>[2x]MAAAAAEEGMEPRALQYEQTLMYGRYTQDLGAFAKEEAARIRLGGPEPWKGPPSSRAAPELLEYGRSRCARCRVCSVRCHKFLVSRVGEDWIFLVLLGLLMALVSWVMDYAIAACLQAQQWMSRGLNTSILLQ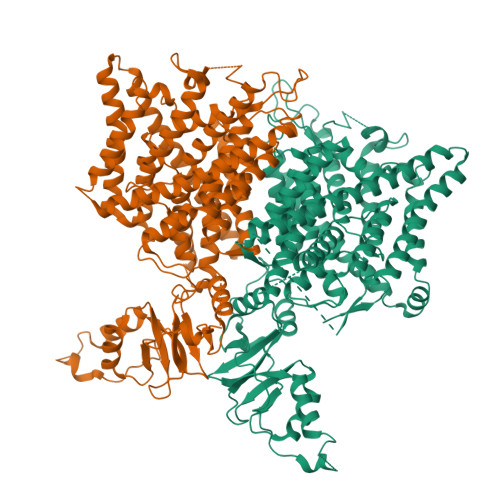YLAWVTYPVVLITFSAGFTQILAPQAVGSGIPEMKTILRGVVLKEYLTLKTFIAKVIGLTCALGSGMPLGKEGPFVHIASMCAALLSKFLSLFGGIYENESRNTEMLAAACAVGVGCCFAAPIGGVLFSIEVTSTFFAVRNYWRGFFAATFSAFIFRVLAVWNRDEETITALFKTRFRLDFPFDLQELPAFAVIGIASGFGGALFVYLNRKIVQVMRKQKTINRFLMRKRLLFPALVTLLISTLTFPPGFGQFMAGQLSQKETLVTLFDNRTWVRQGLVEELEPPSTSQAWNPPRANVFLTLVIFILMKFWMSALATTIPVPCGAFMPVFVIGAAFGRLVGESMAAWFPDGIHTDSSTYRIVPGGYAVVGAAALAGAVTHTVSTAVIVFELTGQIAHILPVMIAVILANAVAQSLQPSLYDSIIRIKKLPYLPELGWGRHQQYRVRVEDIMVRDVPHVALSCTFRDLRLALHRTKGRMLALVESPESMILLGSIERSQVVALLGAQLSPARRRQHMQERRATQTSPLSDQEGPPTPEASVCFQVNTEDSAFPAARGETHKPLKPALKRGPSVTRNLGESPTGSAESAGIALRSLFCGSPPPEAASEKLESCEKRKLKRVRISLASDADLEGEMSPEEILEWEEQQLDEPVNFSDCKIDPAPFQLVERTSLHKTHTIFSLLGVDHAYVTSIGRLIGIVTLKELRKAIEGSVTAQGVKVRPPLASFRDSATSSSDTETTEVHALWGPHSRHGLPREGSPSDSDDKCQ(6M)-N-(2-chloro-4-methylpyridin-3-yl)-6-[4-ethyl-3-(hydroxymethyl)-5-oxo-4,5-dihydro-1H-1,2,4-triazol-1-yl]-5-fluoro-2-{[(2S)-1,1,1-trifluoropropan-2-yl]oxy}pyridine-3-carboxamide | C20 H19 Cl F4 N6 O4 | 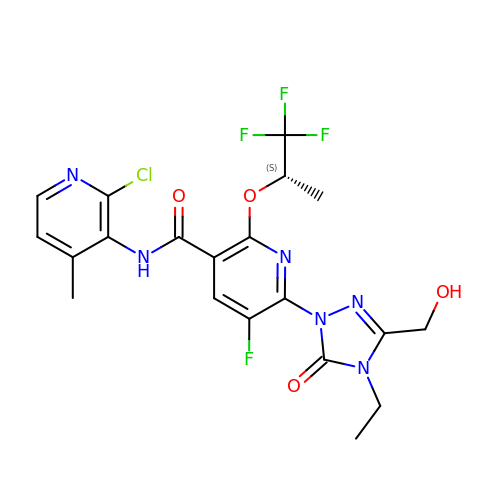XEDJGCIOZDHXOR-JTQLQIEISA-N>[2x]MHHHHHHSWREQGKPPMLF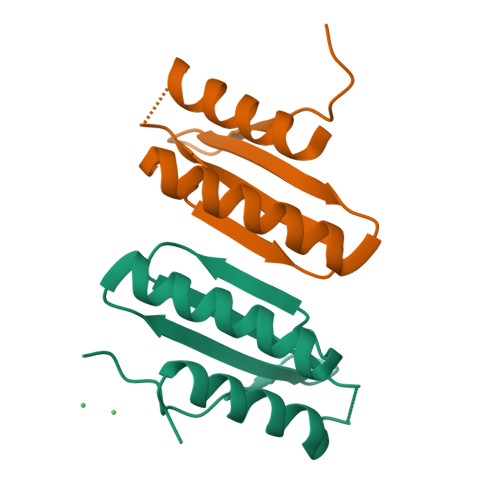KRFAFGSYAQTRAFLDALAALSEETGQHPQNINFGTTYVNITLDAADGATLGEAERAFAARVDALAGSSG>MHHHHHHQQKLTSPDGNLVLTFQVNKEGAPTYDLTYKGKVVIKPSTLGLELKKEDNTRTDFDWVDRRDLTKLDSKSNLYNGFKLKDAQTTTFDETWQPVWGEEKEIRNQYNELAVILFQPMNDRSIVVRFRLFNDGLGFRYEFPQQKSLNYFVIKEEHSQFAMAGNHIAYWIPGDYDTQEYDYTISRLSEIRGLMQQAITPNSSQTPFSPTGVQTALMMKTDDGLYINLHEAALIDYSCMHLNLDDKNMIFESWLTPDAKGDKGYMQTPCNSPWRTIIVSDDARNILASRITLNLNEPCKIADAASWIKPVKYIGVWWDMITGKGSWAYTDELTSVKLGVTDYSKTKPNGKHSANTANVKRYIDFAAANGFDAVLVEGWNEGWEDWFGNSKDYVFDFLTAYPDFDVQEIHRYAASKGIKMMMHHETSASVRNYERHLDKAYQFMVDNGYNSVKSGYVGNIIPRGEHHYGQWMNNHYLYAVKKAADYKIMVNAHEATRPTGICRTYPNLIGNESARGTEYESFGGNKVYHTTILPFTRLVGGPMDYTPGIFETHCNQMNPANNSQVRSTIARQLALYVTMYSPLQMAADIPENYERFMDAFQFIKDVALDWDKTIYLEAEPGEYITIARKAKGTDDWYIGCTAGENGHDSQLTFDFLEPGKQYVATVYADAKDADWKDNPQAYTIKKGILNNKSKLNLHAANGGGYAISIKEVKNKSEVKGLKRL[2x]

Acarbose is a type 2 diabetes medicine that prevents dietary starch breakdown into glucose by inhibiting host amylase and glucosidase enzymes. Species in this phylum normally deploy a well-characterized Starch utilization system (Sus) to recognize, degrade, and import starch. Maltooligosaccharides are transported to the periplasm by a predicted TonB-dependent transporter, SusC, where they are degraded to glucose by a neo-pullulanase/α-amylase, SusA, and an α-glucosidase/glucoamylase, SusB. Instead, we discovered that although acarbose primarily targets the Sus periplasmic GH97 enzymes in both organisms, the drug affects starch processing at multiple other points.

The genes encoding BoGH97CSus (hereafter referred to as BoSusB) and SusB were mutated to introduce a stop codon after eight amino acids, as an in-frame deletion of susB has polar effects in Bt. Furthermore, BoSusB and SusB have similar substrate preferences. Our work here, and previously published work on SusB, demonstrate that both enzymes are exo-acting glucoamylases that accommodate α1,6 and α1,4 linkages and do not break down acarbose. Remarkably, BoSusB had a similar Ki (69 nM). SusB has been structurally characterized and is known to be competitively inhibited by acarbose. We solved a co-crystal structure of BoSusB with acarbose bound in the active site near the dimer interface. Acarbose binds identically to the SusB and BoSusB active sites. The SusRs are 89% identical, and the SusBs are 93% identical between Bo and Bt. Collectively, these data suggest that although BoSusB and SusB drive most of the acarbose phenotype in Bo and Bt, respectively, they are not responsible for the acarbose-induced phenotypic differences.> AQFKEGEHYQVLKTPASSSPVVSEFFSFYCPHCNTFEPIIAQLKQQLPEGAKFQKNHVSFMGGNMGQAMSKAYATMIALEVEDKMVPVMFNRIHTLRKPPKDEQELRQIFLDEGIDAAKFDAAYNGFAVDSMVRRFDKQFQDSGLTG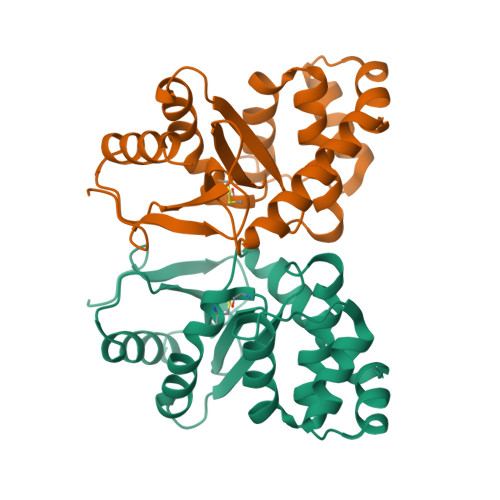VPAVVVNNRYLVQGQSVKSLDEYFDLVNYLLTLK> DSTSTKVIVHYHRFDSNYTNWDVWMWPYQPVNGNGAAYQFTGTNDDFGAVADTQVPGDNTQVGLIVRKNDWSEKNTPNDLHIDLAKGHEVWIVQGDPTIYYNLSDAQAAAIPSVSNAYLDDEKTVLAKLSMPMTLADAASGFTVIDKTTGEKIPVTSAVSANPVTAVLVGDLQQALGAANNWSPDDDHTLLKKINPNLYQLSGT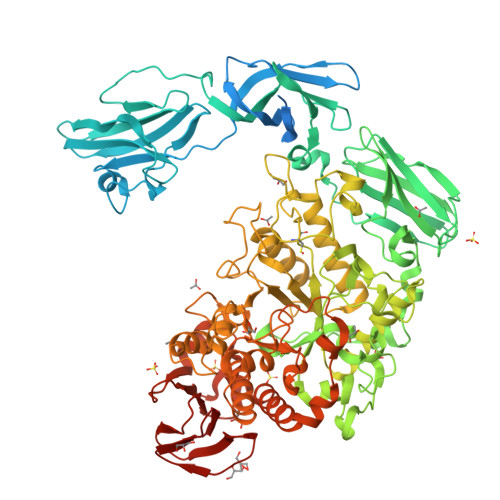LPAGTYQYKIALDHSWNTSYPGNNVSLTVPEGGEKVTFTYIPSTNQVFDSVNHPNQAFPTSSAGVQTNLVQLTLASAPDVTHNLDVAADGYKAHNILPRNVLNLPRYDYSGNDLGNVYSKDATSFRVWAPTASNVQLLLYNSEKGSITKQLEMQKSDNGTWKLQVSGNLENWYYLYQVTVNGTTQTAVDPYARAISVNATRGMIVDLKATDPAGWQGDHEQTPANPVDEVIYEAHVRDFSIDANSGMKNKGKYLAFTEHGTKGPDHVKTGIDSLKELGITTVQLQPVEEFNSIDETQPDTYNWGYDPRNYNVPEGAYATTPEGTARITELKQLIQSLHQQRIGVNMDVVYNHTFDVMVSDFDKIVPQYYYRTDSNGNYTNGSGCGNEFATEHPMAQKFVLDSVNYWVNEYHVDGFRFDLMALLGKDTMAKISNELHAINPGIVLYGEPWTGGTSGLSSDQLVTKGQQKGLGIGVFNDNIRNGLDGNVFDKTAQGFATGDPNQVDVIKNGVIGSIQDFTSAPSETINYVTSHDNMTLWDKILASNPSDTEADRIKMDELAHAVVFTSQGVPFMQGGEEMLRTKGGNDNSYNAGDSVNQFDWSRKAQFKDVFDYFSSMIHLRNQHPAFRMTTADQIKQNLTFLESPTNTVAFELKNYANHDTWKNIIVMYNPNKTSQTLNLPSGDWTIVGLGDQIGEKSLGHVMGNVQVPAISTLILKQ>MHHHHHHHPGFFTSIGQMTDLIHTEKDLVTSLKDYIKAEEDKLEQIKKWAEKLDRLTSTATKDPEGFVGHPVNAFKLMKRLNTEWSELENLVLKDMSDGFISNLTIQRQYFPNDEDQVGAAKALLRLQDTYNLDTDTISKGNLPGVKHKSFLTAEDCFELGKVAYTEADYYHTELWMEQALRQLDEGEISTIDKVSVLDYLSYA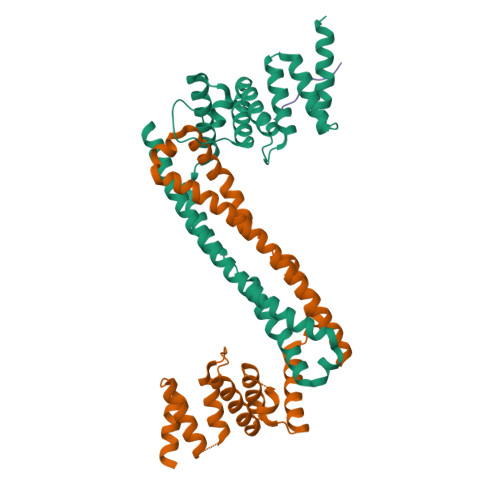VYQQGDLDKALLLTKKLLELDPEHQRANGNLKYFEYIMAKEKDVNKS[2x];> PPGPPGPPG The exosome and its related bacterial polynucleotide phosphorylase (PNPase) represent a class of conserved multi-subunit protein complexes responsible for the 3′-to-5′ processing and degradation of RNA. Architecturally, the ∼250 KDa prototypic archaeal exosome is similar to the bacterial PNPase, consisting of a catalytic ring containing a trimer of Rrp41/Rrp42 heterodimers, and with a trimetric Rrp4 or Csl4 RNA-binding ring stacked on the top. Both Rrp41 and Rrp42 are homologous to RNase PH, but only Rrp41 possesses the phosphorolytic 3′-to-5′ exoribonuclease activity. A large “processing chamber” was found inside the catalytic ring, where three identical phosphorolytic active sites reside.

To further understand the RNA recruitment mechanism of the exosome family of macromolecular machines, we determined the crystal structure of the archaeal Sulfolobus solfataricus exosome. We observed that while the catalytic ring of the S. solfataricus exosome adopts a three-fold symmetric structure, its RNA-binding ring displays considerable rigid body and thermal motions, which broke its internal symmetry. The three copies of Rrp41/Rrp42 heterodimers within the catalytic ring align extremely well with their counterparts in the previous structure, even though the three-fold NCS was not enforced in our structure, the three heterodimers does not deviate notably from their symmetric positions. In addition to rigid body shifts, we observed conformational heterogeneity among Rrp4 subunits. While two of the three copies (Chain C and I) overlap reasonably well with their counterparts in the previous structure, with the r.m.s.d of the Cα alignment at 0.5 Å and 0.6 Å, respectively, and at 0.8 Å with each other, the third Rrp4 copy (Chain F) adopts a significantly different conformation (the r.m.s.d. of 250 Cα alignment is 1.5 Å with the previously published structure). The conformational changes are not due to changes in the crystal packing environment, as minimal crystal contacts were observed around the Rrp4 ring. The exceptionally large geometric deviation in Chain F is due to a rigid body hinge motion at the linker region between the N-terminal domain and the S1/KH domains, because when aligned separately, each domain agrees well with their counterparts in other two Rrp4 subunits (r.m.s.d. of Cα alignments for the N-ter, S1, and KH domains are at 0.3 Å (50 aa), 0.3 Å (70 aa), and 0.7 Å (115 aa), respectively, Fig. 3b–d). The hinge motion causes the S1 and KH domains in chain F to move away from the central channel and thus increases the diameter of the pore opening. Although Chain C and Chain I of Rrp4 adopt very similar conformations, Chain I displays considerably higher thermal motion than Chain C, manifested by a higher average temperature factor of 81 versus 61, as well as wider thermal ellipsoids in Chain I.

>MSSTPSNQNIIPIIKKESIVSLFEKGIRQDGRKLTDYRPLSITLDYAKKADGSALVKLGTTMVLAGTKLEIDKPYEDTPNQGNLIVNVELLPLAYTTFEPGPPDENAIELARVVDRSLRDSKALDLTKLVIEPGKSVWTVWLDVYVLDYGGNVLDACTLASVAALYNTKVYKVEQISVNKNEVVGKLPLNYPVVTISVAKVDKYLVVDPDLDEESIMDAKISFSYTPDLKIVGIQKSGKGSMSLQDIDQAENTARSTAVKLLEELKKHLGI[3x];>MLQVERPKLILDDGKRTDGRKPDELRSIKIELGVLKNADGSAIFEMGNTKAIAAVYGPKEMHPRHLSLPDRAVLRVRYHMTPFSTDERKNPAPSRREIELSKVIREALESAVLVELFPRTAIDVFTEILQADAGSRLVSLMAASLALADAGIPMRDLIAGVAVGKADGVIILDLNETEDMWGEADMPIAMMPSLNQVTLFQLNGSMTPDEFRQAFDLAVKGINIIYNLEREALKSKYVEFKEEGV[3x];>MNMSQSQKIVLQPRSIVVPGELLAEGEFQIPWSPYILKINSKYYSTVVGLFDVKDTQFEVIPLEGSFYYPKINDIVIGLVEDVEIYGWVVDIKAPYKAYLPASNLLGRSINVGEDLRRYLDVGDYVIARIENFDRSIDPVLSVKGKDLGRVSNGIVIDIMPVKVPRVIGKNKSMYETLTSKSGCSIFVANNGRIWATCPSRFSEEILIEAIRKIENESHIKGLTDRIKQFIEEKLGERNASSGETKTNS[3x]> MVKVMLLGDSITEITCWRPLVWEQITSAGLAGSVDFVGSMNDLQPNCSRPQGFDPDHEGHSGWQAYDIARNNIAGWVQNTKPDIVQFMLGTNDVNIG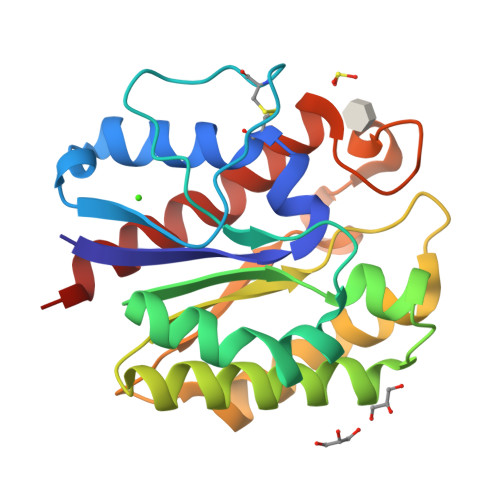HRNADSIIGSYTIMLNAMRAANPRVKVIVDKIIPTSWSDATIEAVNTAIPGWVQQQTTAESPVVIADCSRAAGFTNDMLRDDGVHPNSKGDQFIAGQIGPKLIQLIKDVS>[3x]AQVINTFDGVADYLQTYHKLPDNYITKSEAQALGWVASKGNLADVAPGKSI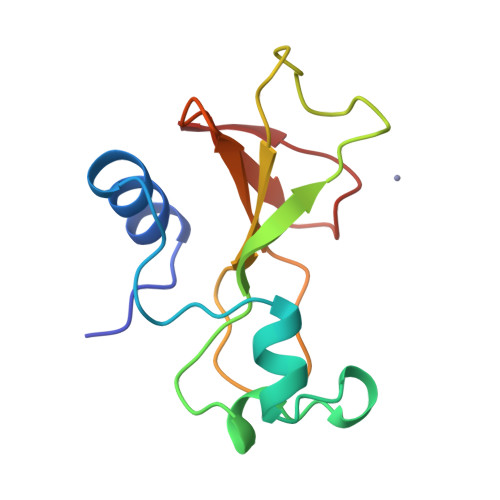GGDIFSNREGKLPGKSGSTWREADINYTSGFRNSDRILYSSDWLIYKTTDHYQTFTKIR> MDYKDDDDKRSPVRDLARNDGEESTDRTPLLPGAPRAEAAPVCCSARYNLAI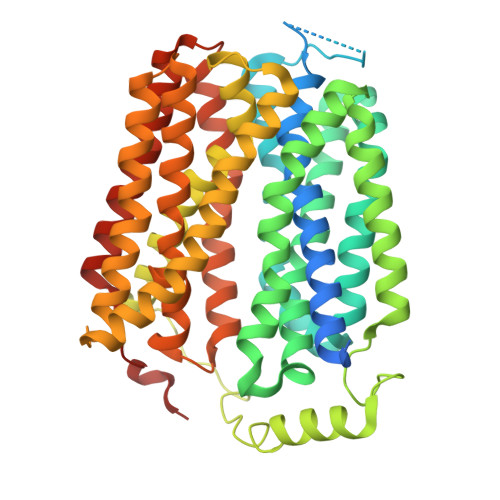LAFFGFFIVYALRVNLSVALVDMVDSNTTLEDNRTSKACPEHSAPIKVHHNQTGKKYQWDAETQGWILGSFFYGYIITQIPGGYVASKIGGKMLLGFGILGTAVLTLFTPIAADLGVGPLIVLRALEGLGEGVTFPAMHAMWSSWAPPLERSKLLSISYAGAQLGTVISLPLSGIICYYMNWTYVFYFFGTIGIFWFLLWIWLVSDTPQKHKRISHYEKEYILSSLRNQLSSQKSVPWVPILKSLPLWAIVVAHFSYNWTFYTLLTLLPTYMKEILRFNVQENGFLSSLPYLGSWLCMILSGQAADNLRAKWNFSTLCVRRIFSLIGMIGPAVFLVAAGFIGCDYSLAVAFLTISTTLGGFCSSGFSINHLDIAPSYAGILLGITNTFATIPGMVGPVIAKSLTPDNTVGEWQTVFYIAAAINVFGAIFFTLFAKGEVQNWALNDHHGHRH> MQEKYKDVLLPKELTQIGDWKVDKNLSDDFNYTTKNKKFFKKWKDSYTNDWTGPGLSHFSSNHSILKDGNLEIKAERKPPNKVYCGVISSRKEVIYPAYMEIKMKISGLKLSSNFWFISKDQVLEIDVNETYGNEPDRSKKMGTNYHIFQRTPFKDLTPNNGKHYTAKGAPFLKDQFHRFGCHWKDAYHADFYLDGTLVRQLTIEDPRTSGVGFNQGLLMV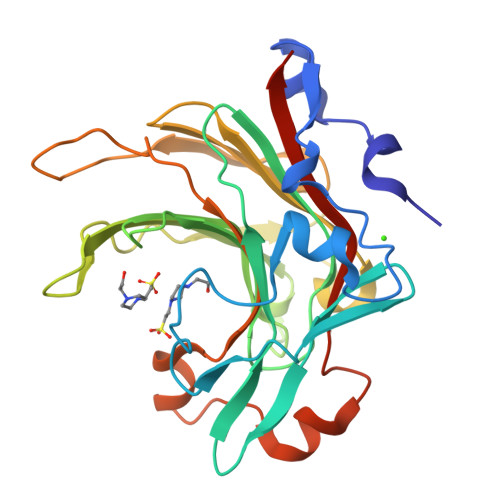IDTEDHDWRSKKGITPTDDELLDETINTMYVDWVRVYKPKLDHHHHHH> GSVRAIDEDCSQYEPIPGSQKAALGYNILTQEDAQSVYDASYYGGQCETVYNGEWRELRYDSTSERLYYGDDEKYFRKPYNFLKYHFEALADTGISSEFYDNANDLLSKVKKDKSDSFGVTIGIGPAGSPLLVGVGVSHSQDTSFLNELNKYNEKKFIFTRIFTKVQTAHFKMRKDDIMLDEGMLQSLMELPDQYNYGMYAKFINDYGTHYITSGSMGGIYEYILVIDKAKMESLGXXXXXXXXXXXXARKAMAVEDIISRVRGGSSGWSGGLAQNRSTITYRSWGRSLKYNPVVIDFEMQPIHEVLRHTSLGPLEAKRQ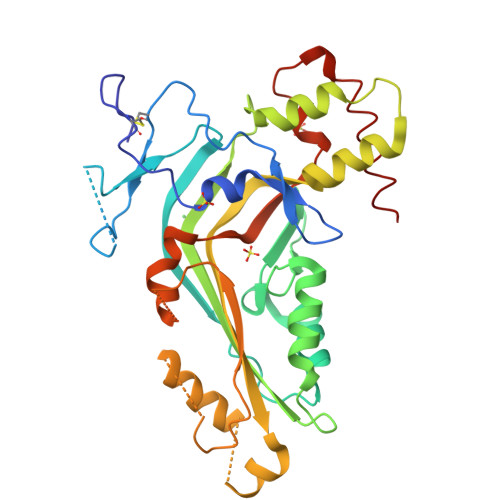NLRRALDQYLMAAA Macrophage-expressed gene 1 (MPEG1, also termed Perforin-2) is one of the most ancient and highly conserved members of the membrane attack complex (MAC)/perforin-like (PF)/cholesterol-dependent cytolysin (MACPF/CDC) superfamily, with orthologous sequences identifiable throughout the metazoan. In contrast to other perforin-like proteins characterised to date, human MPEG1 is an integral type-1 transmembrane protein. The mature protein is comprised of three regions; an ectodomain located in the vesicular lumen, a transmembrane domain anchor that spans the vesicular membrane and, finally, a short cytosolic sequence. Each monomer of the 16-subunit ring possesses an N-terminal MACPF/CDC domain, a central multi-vesicular body of 12 kDa (MVB12)-associated β-prism (MABP) domain and a C-terminal region (termed the L-domain).

Indeed, our (ultimately unsuccessful) attempts to disrupt the interface between the double ring serendipitously led to our identifying the MPEG1 L425K mutation as yielding a greatly improved sample and an improvement in global resolution to 2.4 Å (workflow described in detail in the methods). This mutation resulted in two different MPEG1L425K assemblies, one of which involved domain swapping between the two head-to-head coordinated rings. Three-dimensional classification experiments and multibody analysis of the head-to-head assembly reveal that one ring can adopt multiple positions relative to the other ring, that is, neither ring possesses a single well-defined orientation. In contrast to other MACPF/CDCs studied to date, the recombinant form of MPEG1 has pre-assembled into a soluble oligomer that exhibits the expected features of a prepore assembly. Within each subunit, both TMH-1 and -2 are folded as small helical bundles. A central feature of the assembly is a 64-stranded β-barrel that represents the top, preformed portion of the future pore. The majority of MACPF/CDC domain-mediated inter-subunit interactions are formed around the central lumen of the β-barrel. Around the outside of the assembly both the MABP domain and the L-domain also mediate extensive inter-subunit interactions. The L-domain forms substantial inter-subunit interactions in trans with an extraordinary elongated β-hairpin that extends from the MABP domain of the adjacent subunit (the MABP β-hairpin).

>[32x]KSGKPSGEMDEVGVQKCKNALKLPVLEVLPGGGWDNLRNVDMGRVMELTYSNCRTTEDGQYIIPDEIFTIPQKQSNLEMNSEILESWANYQSSTSYSINTELSLFSKVNGKFSTEFQRMKTLQVKDQAITTRVQVRNLVYTVKINPTLELSSGFRKELLDISDRLENNQTRMATYLAELLVLNYGTHVTTSVDAGAALIQEDHLRASFLQDSQSSRSAVTASAGLAFQNTVNFKFEENYTSQNVLTKSYLSNRTNSRVQSIGGVPFYPGITLQAWQQGITNHLVAIDRSGLPLHFFINPNMLPDLPGPLVKKVSKTVETAVKRYYTFNTYPGCTDLNSPNFNFQANTDDGSCEGKMTNFSFGGVYQECTQLSGNRDVLLCQKLEQKNPLTGDFSCPSGYSPVHLLSQIHEEGYNHLECHRKCTLKVFCKTVCEDVFQVAKAEFRAFWCVASSQVPENSGLLFGGLFSSKSINPMTNAQSCPAGYFPLRLFENLKVCVSQDYELGSRFAVPFGGFFSCTVGNPLVDPAISRDLGAPSLKKCPGGFSQHPALISDGCQVSYCVKSGLFTGGSLPPARLPPFTRPPLMSQAATNTVIVTNSENARSWIKDSQTHQWRLGEPIELRRAMNVIHGDGGGLSHHHHHH> VDC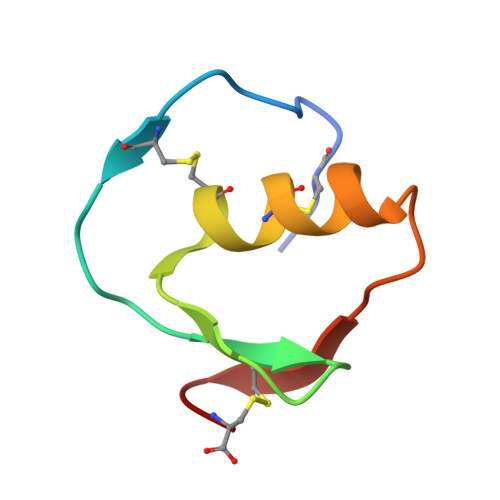SEYPKPACTHEYRPLCGSDNKTYGNKCNFCNAVVESNGTLTLSHFGKC>SEKSEEINEKDLRKKSELQGTALGNLKQIYYYNEKAKTENKESHDQFLQHTILFKGFFTDHSWYNDLLVDFDSKDIVDKYKGKKVDLYGAYYGYQCAGGTPNKTACMYGGVTLHDNNRLTEEKKVPINLWLDGKQNTVPLETVKTNKKNVTVQELDLQ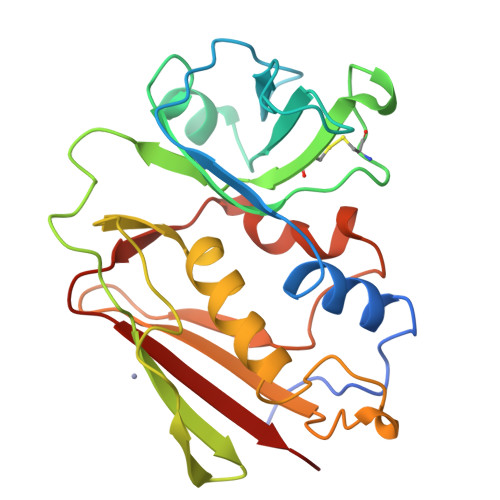ARRYLQEKYNLYNSDVFDGKVQRGLIVFHTSTEPSVNYDLFGAQGQYSNTLLRIYRDNKTINSENMHIDIYLYTS[2x]>MGSSHHHHHHGSPIHDKSPRPQEFAAVDLGSNSFHMVIARVVDGAMQIIGRLKQRVHLADGLGPDNMLSEEAMTRGLNCLSLFAERLQGFSPASVCIVGTHTLRQALNATDFLKRAEKVIPYPIEIISGNEEARLIFMGVEHTQPEKGRKLVIDIGGGSTELVIGENFEPILVESRRMGCVSFAQLYFPGGVINKENFQRARMAAAQKLETLTWQFRIQGWNVAMGASGTIKAAHEVLMEMGEKDGIITPERLEKLVKEVLRHRNFASLSLPGLSEERKTVFVPGLAILCGVFDALAIRELRLSDGALREGVLYEMEGRFRHQDVRSRTASSLANQYHIDSEQARRVLDTTMQMYEQWREQQPKLAHPQLEALLRWAAMLHEVGLNINHSGLHRHSAYILQNSDLPGFNQEQQL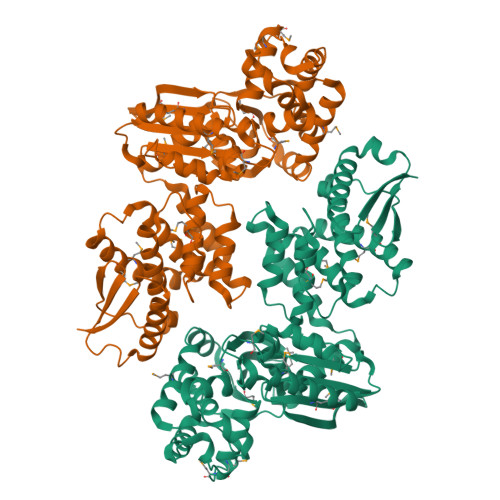MMATLVRYHRKAIKLDDLPRFTLFKKKQFLPLIQLLRLGVLLNNQRQATTTPPTLTLITDDSHWTLRFPHDWFSQNALVLLDLEKEQEYWEGVAGWRLKIEEESTPEIAA[4x]> ASTAPVADHKGRVGHVSQVIGAVVDVHFADGVPPVLTALDVV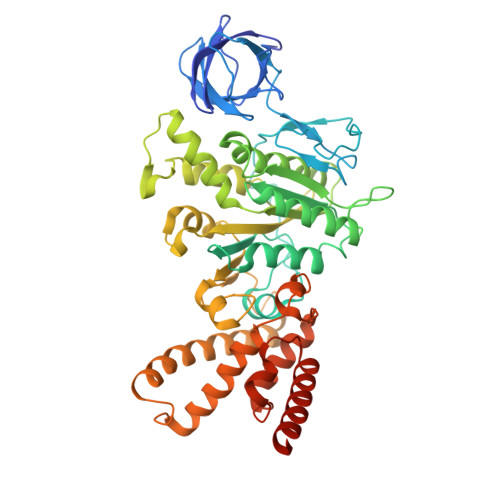DKLGRDEPLTLEIVQHLDAHTGRCIAMQTTDLLKLKAKVVSTGGNISVPVGRETLGRIFNVLGDAIDQRGPVGEKLRMPIHAVAPKLADQAAEDAVLTTGIKVIDLILPYCKGGKIGLFGGAGVGKTVIIMELINNVAKGHGGFSVFAGVGERTREGTDLYLEMMQSKVIDLKGESKCVLVYGQMNEPPGARARVAQSALTMAEYFRDVEGQDVLLFIDNIFRFTQANSEVSALLGRIPAAVGYQPTLAEDLGQLQERITSTTKGSITSVQAVYVPADDITDPAPATTFSHLDATTVLDRAVAESGIYPAVNPLECASRIMDPDVISVDHYNVAQDVVQMLTKYRELQDIIAVLGIDELSEEDKLIVDRARKLVKFLSQPFQVAEVFTGMTGHYVQLDDTIDSFSGLLMGTYDQVPEMAFYMVGGINSVLEKAKKMAEEAAELEKMRRARVAQASS>TSHHHHHMKKIEHKMVAVNGLNMHLAELGEGPTILFIHGFPELWYSWRHQMVYLAERGYRAVAPDLRGYGDTTGAPLNDPSKFSILHLVGDVVALLEAIAPNEEKVFVV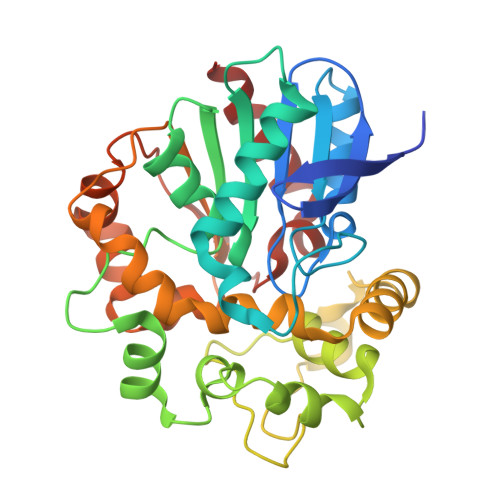AHDWGALIAWHLCLFRPDKVKALVNLSVHFSKRNPKMNVVEGLKAIYGEDHYISRFQVPGEIEAEFAPIGAKSVLKKILTYRDPAPFYFPKGKGLEAIPDAPVALSSWLSEEELDYYANKFEQTGFTGAVNYYRALPINWELTAPWTGAQVKVPTKFIVGEFDLVYHIPGAKEYIHNGGFKKDVPLLEEVVVLEGAANFVSQERPHEISKHIYDFIQKF[2x]> VPRMPVFHTRTIESILEPVAQQISHLVIMHEEGEVDGKAIPDLTAPVSAVQAAVSNLVRVGKETVQTTEDQILKRDMPPAFIKVENACTKLVRAAQMLQADPYSVPARDYLIDGSRGILSGTSDLLLTFDEAEVRKIIRVCKGILEYLTVAEVVETMEDLVTYTKNLGPGMTKMAKMIDERQQELTHQEHRVMLVNSMNTVKELLPVLISAMKIFVTTKNTKSQGIEEALKNRNFTVEKMSAEINEIIRVLQLTSWDEDAWASKDTEAMKRALALIDSKMNQAK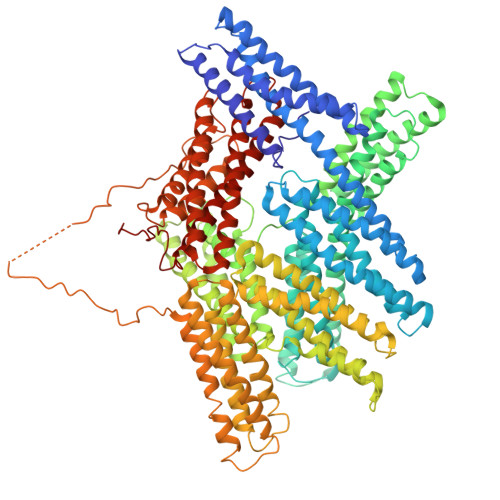GWLRDPNAPPGDAGEQAIRQILDEAGKAGELCAGKERREILGTCKTLGQMTDQLADLRARGQGATPMAMQKAQQVSQGLDLLTAKVENAARKLEAMTNSKQAIAKKIDAAQNWLADPNGGSEGEEHIRGIMSEARKVAELCEEPKERDDILRSLGEISALTAKLSDLRRHGKGDSPEARALAKQIATSLQNLQSKTNRAVANTRPVKAAVHLEGKIEQAQRWIDNPTVDDRGVGQAAIRGLVAEGRRLANVMMGPYRQDLLAKCDRVDQLAAQLADLAARGEGESPQARAIAAQLQDSLKDLKARMQEAMTQEVSDVFSDTTTPIKLLAVAATAPSDTPNREEVFEERAANFENHAARLGATAEKAAAVGTANKTTVEGIQATVKSARELTPQVVSAARILLRNPGNQAAYEHFETMKNQWIDNVEKMTGLVDEAIDTKSLLDASEEAIKKDLDKCKVAMANMQPQMLVAGATSIARRANRILLVAKREVENSEDPKFREAVKAASDELSKTISPMVMDAKAVAGNISDPGLQKSFLDSGYRILGAVAKVREAFQPQEPDFPPPPPDLEHLHLTDELAPPKPPLPEGEVPPPRPPPPEEKDEEFPEQKAGEAINQPMMMAARQLHDEARKWSSKGNDIIAAAKRMALLMAEMSRLVRGGSGNKRALIQCAKDIAKASDEVTRLAKEVAKQCTDKRIRTNLLQVCERIPTISTQLKILSTVKATMLGRTNISDEESEQATEMLVHNAQNLMQSVKETVREAEAASIKIRTDAGFTLRWVRKTPWYQ>MASDAQAGPAPSRDDRVDRQPRLPAAPRVAEVGLNAPSVDYPFQWVVASYDGSEAKNLSDDLSGSATLTKVMANYRHAELTSVELEVCPLAAAFSKPISVSAVWTIASISPASASETSYYGGRLFTVGGPVLMSSTTHLPADLTRLNPVLKGPVKYTDCPRFSYSVYSNGGTKGTNLCTIILRGVVRLSGPSGNLLA[3x]

CSDaV is a positive-sense, single-stranded RNA virus that belongs to the genus Marafivirus in the family Tymoviridae and has a monopartite genome of about 6.8 Kb. In brief, CSDaV encodes for three quasi-equivalent CPs that share amino acid (aa) sequences at the C-terminus but differ from each other at the N-terminus. The whole capsid models of the two types of particles are almost indistinguishable and reveals a T = 3 icosahedral symmetry that gives particles with a diameter of about 30 nm. Each subunit of the asymmetric unit has typical Jelly Roll folds which consist of eight antiparallel beta sheets.

Sodium dodecyl sulfate-polyacrylamide gel electrophoresis (SDS-PAGE) densitometry analysis of purified wild-type (WT)-CSDaV virions showed that > 80% of the CP subunits are composed of the CPp21, while the other < 20% are composed of the CPp23 and CPp25 together, indicating higher expression of CPp21 over the other two CP subunits. The major CP (CPp21) is a product of direct translation from the second start codon in the CSDaV subgenomic RNA (sgRNA), whereas the minor CPs, CPp25 and CPp23, are produced respectively by direct translation from the first start codon in the sgRNA and by proteolytic cleavage processing of the p25 precursor. In attempts to reveal where (if in the inside or outside) GFP is displayed on the GFP-recombinant CSDaV virions (CS-GFPdupCS), we have determined the cryo-EM structures of both the WT- and the CS-GFPdupCS-derived virions. In total, 175,869 and 12,732 particles were used for structure reconstruction of WT and CS-GFPdupCS virions, respectively, yielding density maps at a resolution of 3.1 Å for WT and 3.4 Å for CS-GFPdupCS virus (see Table S2 for refinement statistics). The primary sequence of the CSDaV major CP (CPp21) was used to generate initial models (by automated homology modeling) for the WT and CS-GFPdupCS virions. Both final models were built as a single asymmetric unit that comprises three chains (A, B, and C). Analysis comparing our results with protein domain structure annotations available in the CATH database, revealed that the CSDaV capsid has similar subunit arrangement and tertiary structure with desmodium yellow mottle tymovirus (DYMV), in which chain A forms pentameric capsomeres while chains B and C form hexametric capsomeres. Residues 1−65 were not visible for the CSDaV WT CPs, while residues 1−276 (including the full aa sequence of the GFP) were not visible for the GFP-fused CP (respectively). However, analysis on the position of each asymmetric unit chain in the capsid of WT-CSDaV particles indicates that the N-terminal region of the CPs is displayed towards the inside of the particle, whereas the C-terminal region is directed to the outside surface of the particle. This might indicate that the N-terminal region, non-visible in the electron density map, could potentially be hidden inside of the particle.> MDTTVPTFSLAELQQGLHQDEFRRCLRDKGLFYLTDCGLTDTELKSAKDLVIDFFEHGSEAEKRAVTSPVPTMRRGFTGLESESTAQITNTGSYSDYSMCYSMGTADNLFPSGDFERIWTQYFDRQYTASRAVAREVLRATGTEPDGGVEAFLDCEPLLRFRYFPQVPEHRSAEEQPLRMAPHYDLSMVTLIQQTPCANGFVSLQAEVGGAFTDLPYRPDAVLVFCGAIATLVTGGQVKAPRHHVAAPRRDQIAGSSRTSSVFFLRPNADFT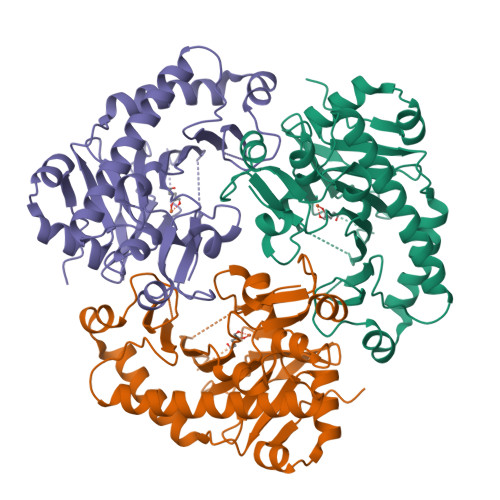FSVPLARECGFDVSLDGETATFQDWIGGNYVNIRRTSKA>[2x]MVFRKSLLKLAVFALGACVAFSNANAAEGKLESIKSKGQLIVGVKNDVPHYALLDQATGEIKGFEVDVAKLLAKSILGDDKKIKLVAVNAKTRGPLLDNGSVDAVIATFTITPERKRIYNFSEPYYQDAIGLLVLKEKKYKSLADMKGANIGVAQAATTKKAIGEAAKKIGIDVKFSEFPDYPSIKAALDAKRVDAFSVDKSILLGYVDDKSEILPDSFEPQSY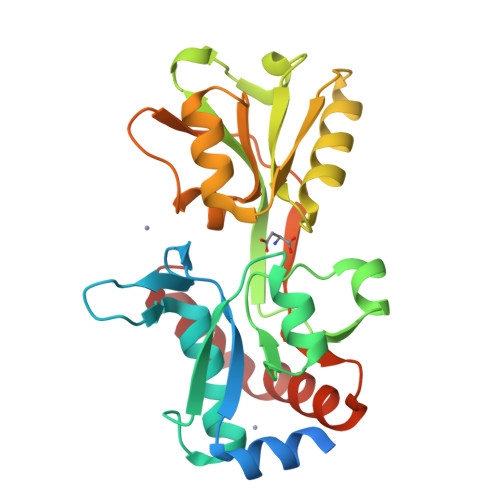GIVTKKDDPAFAKYVDDFVKEHKNEIDALAKKWGL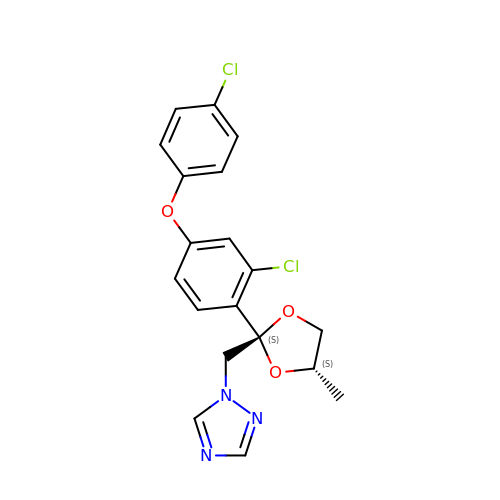1-[[(2~{S},4~{S})-2-[2-chloranyl-4-(4-chloranylphenoxy)phenyl]-4-methyl-1,3-dioxolan-2-yl]methyl]-1,2,4-triazole | C19 H17 Cl2 N3 O3 | BQYJATMQXGBDHF-ORAYPTAESA-N>[2x]MTMEQFLTSLDMIRSGCAPKFKLKTEDLDRLRVGDFNFPPSQDLMCYTKCVSLMAGAVNKKGEFNAPKALAQLPHLVPPEMMEMSRKSVEACRDTHK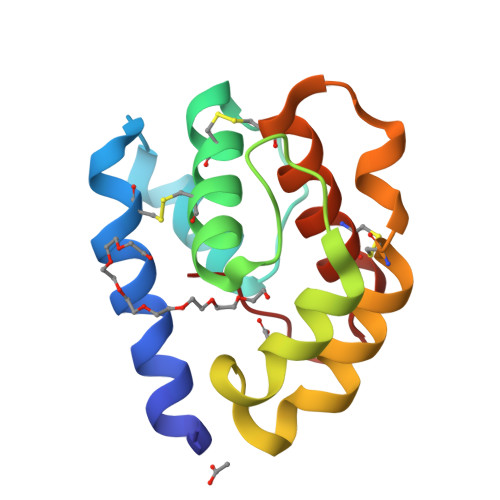QFKESCERVYQTAKCFSENADGQFMWP6-azanyl-11-methyl-2-oxidanylidene-7-[[(2R)-oxolan-2-yl]methyl]-N-(pyridin-3-ylmethyl)-1,9-diaza-7-azoniatricyclo[8.4.0.0^{3,8}]tetradeca-3(8),4,6,9,11,13-hexaene-5-carboxamide | C24 H25 N6 O3 | 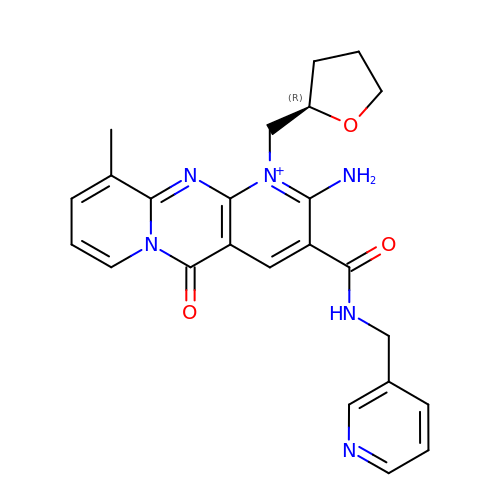XPXWHWPEIBBBCJ-QGZVFWFLSA-O5-[7-(difluoromethyl)-6-(1-methyl-1H-pyrazol-4-yl)-3,4-dihydroquinolin-1(2H)-yl]-N-methyl-1H-indole-3-carboxamide | C24 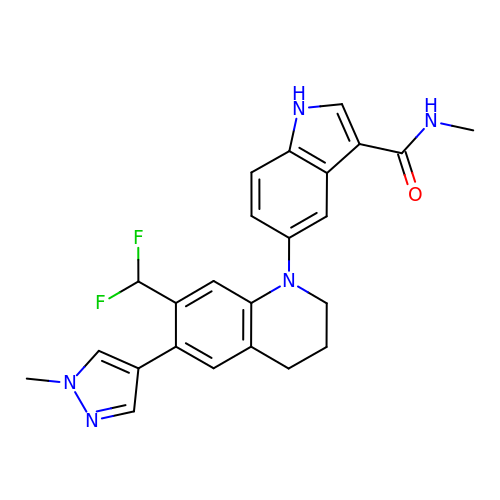H23 F2 N5 O | PQVUDEGEQFDCRY-UHFFFAOYSA-N> MDKSKNIANLVFNGNPRIQLMKDNLFKEERQISLERALLYTESYQQTEGEPVIIRRAKAIQHILENVQISIREGELLAGNRTVRPRSGILSPEMDPYWIVKEIDTIATRPQDQFVFTEADKKIYMEKLYPYWEGRSMKDFINAQLTDDVQQAMTDEVFKLNQTDKGQGHIIMDFPAILEHGVQYYIDILSDKITEQPDNHFFKAGYLICQAMKDHFIRYADLAQEMSLTADACRRQELERIAQMCYKLSQEKPDSFYEALQLLWMTSIVAQYESNASSLSLGRTDQYLYPFYKASLEAGESEAFMYEALGDFYIKTNDVVLLRSQSSAKCFAGFPTGYTIALGGLDEYGHTAVNPLSYIMLDIYHEILLPQPNLSVRMNELIPRRFLLKTCETIRLGTGIPQLFNDEVCVPAFLSKGVSLDDARDYATVGCVETSIPGRTYGLHDIALFNLLRIMELSLYDLRYQTQVTYQDIWKDIEAKIDYYVNLVVKGSNIVDLGHRHYAPTPFLSLLIADCLKNGKDVTEGGARYNFSGVQGIGQANLSDSMYVVQKLVFEQHEMTLAELVDALEANYEGKYVNLQKHVIQDFDKYGNDNDDVDDIAVKLFRHY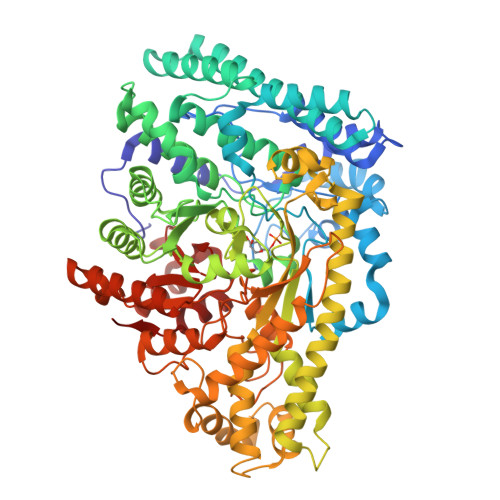AKELEKYENVRGGRFIPGAYTVSAHIPLGEAVGATPDGRKAKEQLADGGLSPMVGRDHLGPTAVLKSVSKLDNYLTVNGSLLNVKFQPNTLKGIEGLTKFADFLMAYTKLKIQHIQFNVQSKATLLDAQKHPEKYTGLLVRVAGYSAFFVDLNKQIQDDIIARVEHQL> MSTQREYVFIPITNSITIDVKITIGGSDHITNIDERGIHNVLVITGYAVDEKNGRLVPTLDPCDYVKG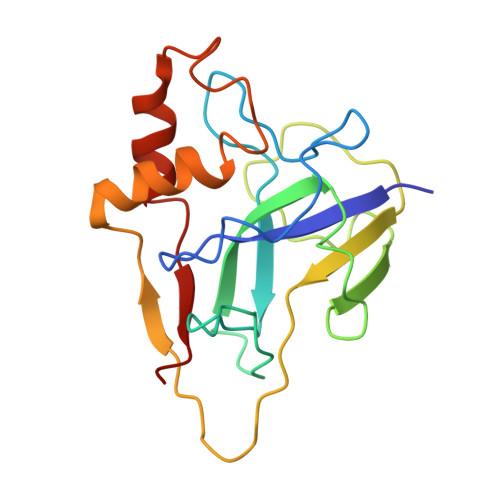ILVAGTPQQAQSNDFLTLKLPANKLYLIRKKGNISDDLKIYIPYSSPDARNSMKTKPVSISDDTIVNNIIKEVFDKIYNITQKEKVKIEKVKEDIKELFSYYALEQ> GSLHCPAACTCSNNIVDCRGKGLTEIPTNLPETITEIRLEQNTIKVIPPGAFSPYKKLRRIDLSNNQISELAPDAFQGLRSLNSLVLYGNKITELPKSLFEGLFSLQLLLLNANKINCLRVD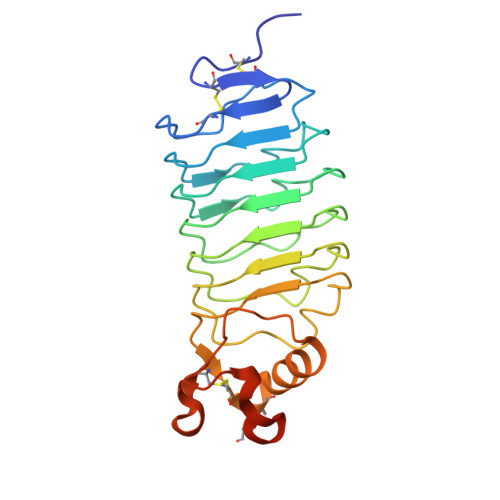AFQDLHNLNLLSLYDNKLQTIAKGTFSPLRAIQTMHLAQNPFICDCHLKWLADYLHTNPIETSGARCTSPRRLANKRIGQIKSKKFRCSAAAHHHHHH> MLADGFETDIAIPSGISRPDAAALQRCEGRVVFLPTIRRQLTLADVAHESFVSGGVSPDTLGLLLAYRRRFPAVITRVLPTRIVACPLDVGLTHAGTVNLRNTSPVDLCNGDPISLVPPVFEGQATDVRLDSLDLTLRFPVPLPSPLAREIVARLVARGIRDLNPSPRNPGGLPDLNVLYYNGSRLSLLADVQQLGPVNAELRSL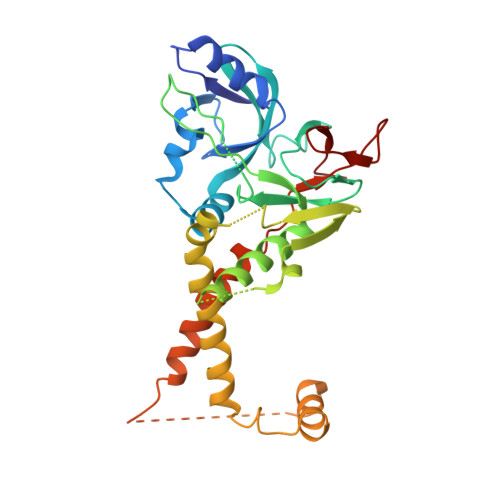VLNMVYSITEGTTIILTLIPRLFALSAQDGYVNALLQMQSVTREAAQLIHPEAPALMQDGERRLPLYEALVAWLTHAGQLGDTLALAPVVRVCTFDGAAVVRSGDMAPVIRYP>MVPTQAHPEWYKSAVFYELSVRTFQDGNGDGKGDFPGLTSRLDYLKNLGVDCLWLLPWFPSPLRDDGYDVADYRGIHPDLGTLDDFKVFLREAHARGLWVIGDLVTNHTSSDHPWFQAARRGPTLPDGSPNEYHDYYVWSDEGKEYADTRIIFTDTEVSNWTLDEQAGKYYWHRFFASQPDLNYDNPKVVEELHGAARFWLDLGLDGFRVDAVPYLIEREGTSCENLPETHEILKGFRAMVDREYPGRLLLAEARQWPEEVVEYFGTEAEPEFHMCFNFPVMPRLYMSLKREDTSSIRE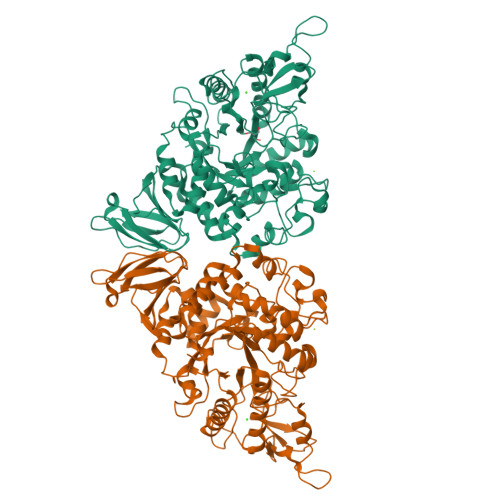IMGRLPKIPSFGQWCIFLRNHDELTLEMVTDDERAFMYAAYAPDARMKINVGIRRRLAPLLDNDRRRIELLNTVLLALPGSPVLYYGDEIGMGDDLGLPDRNGVRTPMQWNAGTSGGFSTAQPSDCFFPPIQDPVYGFGRVNVQSQLQDPSSLLKWTARQLELRRAHPAFAHGDLTFIETGNPAILAFTRQYDGETLLIVSNFAGNAQAGLLDLAPFVGRAPVTLSGASPLPVVTGNGQYPVVMGKYDYYWLRLNSRVDKLAAALEHHHHHH[4x]> GPMTDQAFVTLTTNDAYAKGALVLGSSLKQHRTTRRLVVLATPQVSDSMRKVLETVFDEVIMVDVLDSGDSAHLTLMKRPELGVTLTKLHCWSLTQYSKCVFMDADTLVLANIDDLFDREELSAAPDPGWPDCFNSGVFVYQPSVETYNQLLHLASEQGSFDGGDQGILN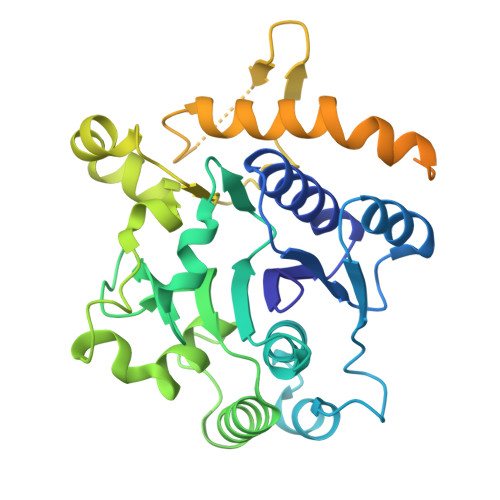TFFSSWATTDIRKHLPFIYNLSSISIFSYLPAFKVFGASAKVVHFLGRVKPWNYTYDPKTKSVKSEAHDPNMTHPEFLILWWNIFTTNVLPLLQQFGLVKDTCSYVNVLSDLVYTLAFSCGFCRKEDVSGAISHLSLGEIPAMAQPFVSSEERKERWEQGQADYMGADSFDNIKRKLDTYLQ N~1~-[2-(1H-indazol-5-yl)pyrido[3,4-d]pyrimidin-4-yl]-2-methylpropane-1,2-diamine | C18 H19 N7 | 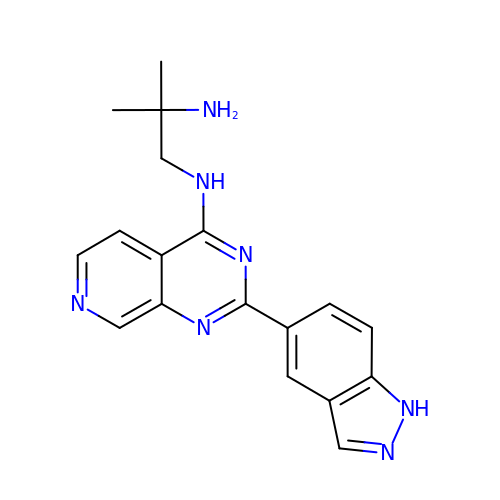PTOPXBFSXASLNA-UHFFFAOYSA-N>[2x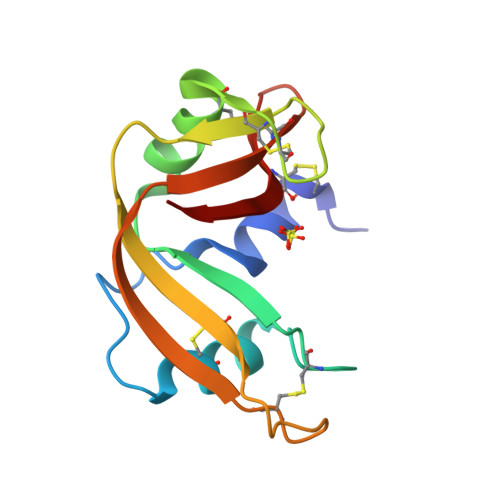]KETCAAKFERQHMDSSTSAASSSNYCNQMMKSRNLTKDRCKPVNTFVHESLADVQAVCSQKNVACKNGQTNCYQSYSTMSITECRETGSSKYPNCAYKTTQANKHIIVACEGNPYVPCHFDASV>EFHMEQKTPKESDRCGGCGKFTHEDDLIALEEEKKKEKEKPLMSKKKSHHHKKNDFQWIGCDSCQTWYHFLCSGLEQFEYYLYEKFFCPKCVPHTGHSIRYKVVAPHRYRWYSPNEKHLGIEVGSKTWIEDFITRENTVPSPTDDEVCIVEDGYEFRREFEKLGGADNWGKVFMVKDMDGLNMTMPKPGFDLEDVVKIMGSDYEVDTIDVYNQSTYSMKLDTFRKLFRDTKNRPLLYNFLSLEFSDNNEMKEIAKPPRFVQEISMVNRLWPDVSGAEYIKLLQREEYLPEDQRPKVEQFCLAGMAGSYTDFHVDFGGSSVYYHILKGEKIFYIAAPTEQNFAAYQAHETSPDTTTWFGDIANGAVKRVVIKEGQTLLIPAGWIHAVLTPVDSLVFGGNFLHLGNLE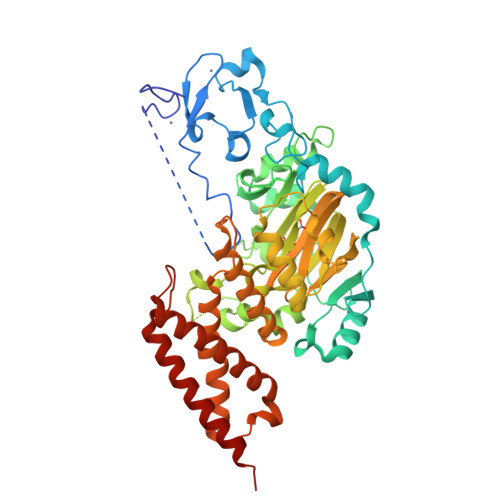MQMRVYHLENAIRKEIRSEEKFYFPNFELLHWMYMRNVLLEKITEANQEGSDMREQEKNIWTASQIMKAEMERWMDRELRLGPEKNAILPTDDKNKIMISVRKQIEIQTKIQNAKNKPMGLK[2x]>[2x]MSNEVEQKKNIKTINDLPGISQTVINKLIEAGYSSLETLAVASPQDLSVAAGIPLSTAQKIIKEARDALDIRFKTALEVKKERMNVKKISTGSQALDGLLAGGIETRTMTEFFGEFGSGKTQLCHQLS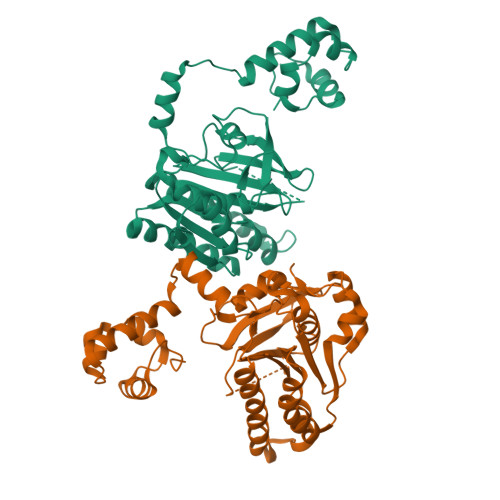VNVQLPPEKGGLSGKAVYIDTEGTFRWERIENMAKALGLDIDNVMNNIYYIRAINTDHQIAIVDDLQELVSKDPSIKLIVVDSVTSHFRAEYPGRENLAVRQQKLNKHLHQLTRLAEVYDIAVIITNQVMARPDMFYGDPTVAVGGHTLYHVPGIRIQLKKSRGNRRIARVVDAPHLPEGEVVFALTEEGIRDAEE>MTEGSVARQPDLSTCDDEPIHIPGAIQPHGLLLALAADMTIVAGSDNLPELTGLAIGALIGRSAADVFDSETHNRLTIALAEPGAAVGAPIAVGFTMRKDAGFVGSWHRHDQLVFLELEPPQRDVAEPQAFFRRTNSAIRRLQAAETLESACAAAAQEVREITGFDRVMIYRFASDFSGEVIAEDRCAEVESYLGLHFPASDIPAQARRLYTINPVRIIPDINYRP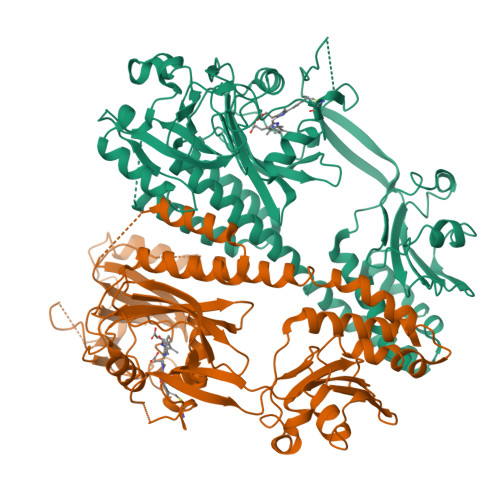VPVTPDLNPVTGRPIDLSFAILRSVSPVHLEYMRNIGMHGTMSISILRGERLWGLIACHHRKPNYVDLDGRQACELVAQVLAWQIGVMEEQAITRQTLKGQAIQRSLINDIEQLHDHRAGLARNSEALLELMGASGLCLHSREGVITIGQTPPGPIIDQLAQLAGRSGGSELFQTDRLSTIIPEAGAFAEVASGVLAVPLSRTPPRRVMLWFRPEVAQTVYWAGNPDKSVTAESGRLRPRTSFAAWTEQTHGRAIAWQPHEVAAAVEIRDLIIDVILRNTKLAAALEHHHHHH[2x]>EKKKADIVFLLDGSINFRRDSFQEVLRFVSEIVDTVYEDGDSIQVGLVQYNSDPTDEFFLKDFSTKRQIIDAINKVVYKGGRHANTKVGLEHLRVNHFVPEAGSRLDQRVPQIAFVITGGKSVEDAQDVSLALTQRGVKVFAVGVRNIDSEEVGKIASNSATAFRVGNVQELSELSEQVLETLH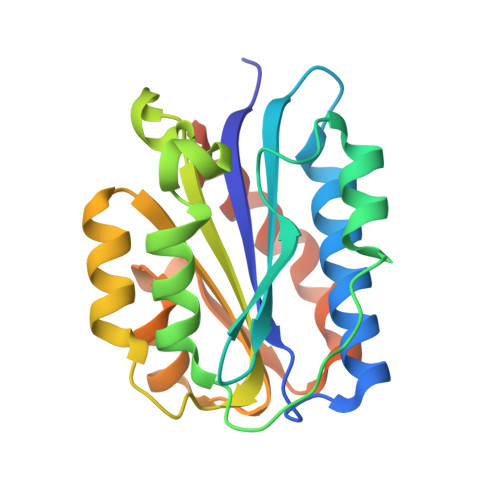DAMHETLCPGVTDAAK[2x]>[2x]SHPDLNKLLELWPHIQEYQDLALKHGINDIFQDNGGKLLQVLLITGLTVLPGREGNDAVDNAGQEYELKSINIDLTKGFSTHHHMNPVIIAKYRQVPWIFAIYRGIAIEAIYRLEPKDLEFYYD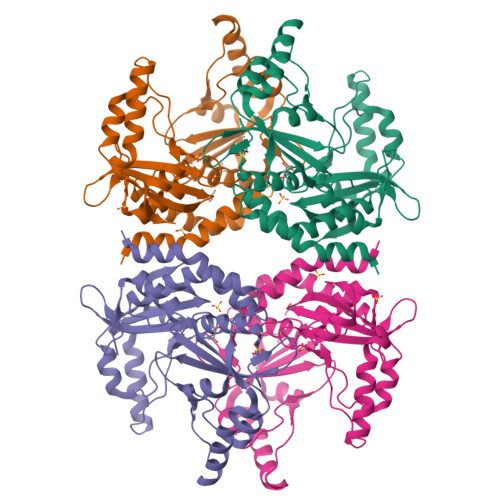KWERKWYSDGHKDINNPKIPVKYVMEHGTKIYGSGGSHPDLNKLLELWPHIQEYQDLALKHGINDIFQDNGGKLLQVLLITGLTVLPGREGNDAVDNAGQEYELKSINIDLTKGFSTHHHMNPVIIAKYRQVPWIFAIYRGIAIEAIYRLEPKDLEFYYDKWERKWYSDGHKDINNPKIPVKYVMEHGTKIYGSHHHHHH> VVWTDFERATIADIFSKLDYEAVGGATL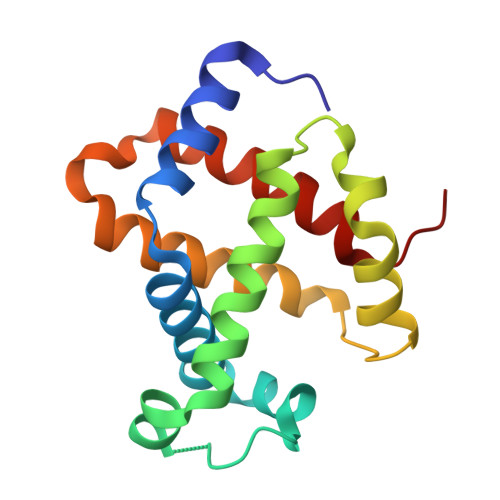ARCLIVYPWTQRYFGNFGNLYNAAAIMGNPMIAKHGTTILHGLDRAVKNMDNIKATYAELSVLHSEKLHVDPDNFKLLSDCLTIVVAAQLGKAFSGEVQAAFQKFLSVVVSALGKQYH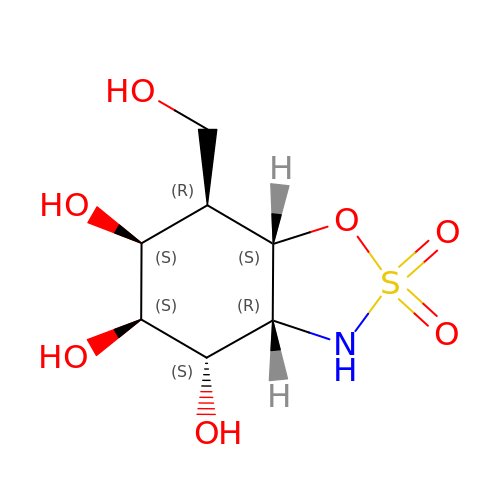(3~{a}~{R},4~{S},5~{S},6~{S},7~{R},7~{a}~{S})-7-(hydroxymethyl)-2,2-bis(oxidanylidene)-3~{a},4,5,6,7,7~{a}-hexahydro-3~{H}-benzo[d][1,2,3]oxathiazole-4,5,6-triol | C7 H13 N O7 S | LDXSPHJOJCEWFB-MREPKMFUSA-N>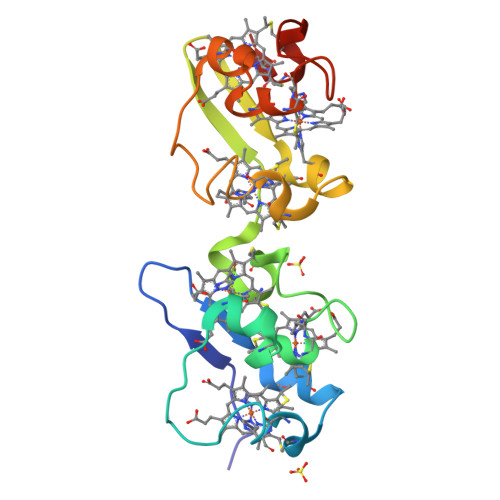 MTPPKTVNFKMKGVADAAFSHEFHLGMYKCNECHTKLFAYKAGAKRFTMADMDKGKSCGACHNGKDAFSSASDCGKCHPGLKPAKLTYKTSVGEAYFDHDIHLSMFKCADCHTKVFKYRKGSAPATMADMEKGKSCGVCHNGKDAFSVADDCVKCHNM>NVSLQPPPQQLIVQNKTIDLPAVYQLNGGEEANPHAVKVLKELLSGKQSSKKGMLISIGEKGDKSVRKYSRQIPDHKEGYYLSVNEKEIVLAGNDERGTYYALQTFAQLLKDGKLPEVEIKDYPSVRYRGVVEGFYGTPWSHQARLSQLKFYGKNKMNTYIYGPKDDPYHSAPNWRLPYPDKEAAQLQELVAVANENEVDFVWAIHPGQDIKWNKEDRDLLLAKFEKMYQLGVRSFAVFFDDISGEGTNPQKQAELLNYIDEKFAQVKPDINQLVMCPTEYNKSWSNPNGNYLTTLGDKLNPSIQIMWTGDRVISDITRDGISWINERIKRPAYIWWNFPVSDYVRDHLLLGPVYGNDTTIAKEMSGFVTNPMEHAESSKIAIYSVASYAWNPAKYDTWQTWKDAIRTILPSAAEELECFAMHNSDLGPNGHGYRREESMDIQPAAERFLKAFKEGKNYDKADFETLQYTFERMKESADILLMNTENKPLIVEITPWVHQFKLTAEMGEEVLKMVEGRNESYFLRKYNHVKALQQQMFYIDQTSNQNPYQPGVKTATRVIKPLIDRTFATVVKFFNQKFNAHLDATTDYMPHKMISNVEQIKNLPLQVKANRVLISPANEVVKWAAGNSVEIELDAIYPGENIQINFGKDAPCTWGRLEISTDGKEWKTVDLKQKESRLSAGLQKAPVKFVRFTNVSDEEQQVYLRQFVLTIEKK[2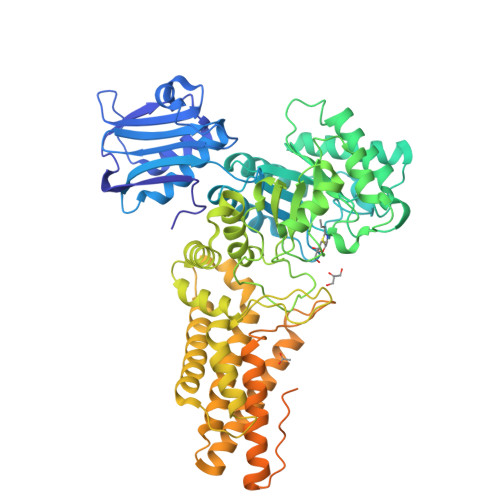x]> Q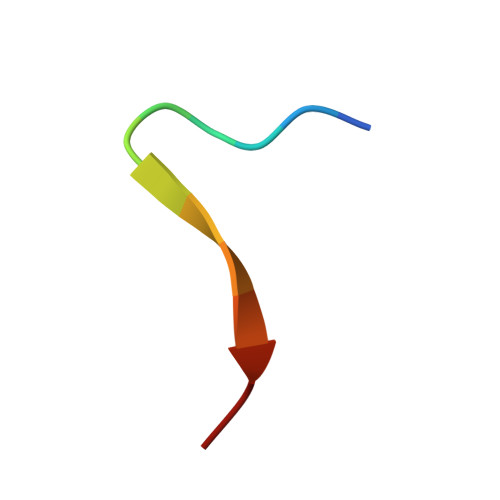KAPPGTARRKRK>[4x]MAKKTSSKGKLPPGPTPLPFIGNYLQLNTEQMYNSLMKISERYGPVFTIHLGPRRVVVLCGHDAVREALVDQAEEFSGRGEQATFDWVFKGYGVVFSNGERAKQLRRFSIATLRDFGVGKRGIEERIQEEAGFLIDALRGTGGANIDPTFFLSRTVSNVISSIVFGDRFDYKDKEFLSLLRMMLGIFQFTSTSTGQLYEMFSSVM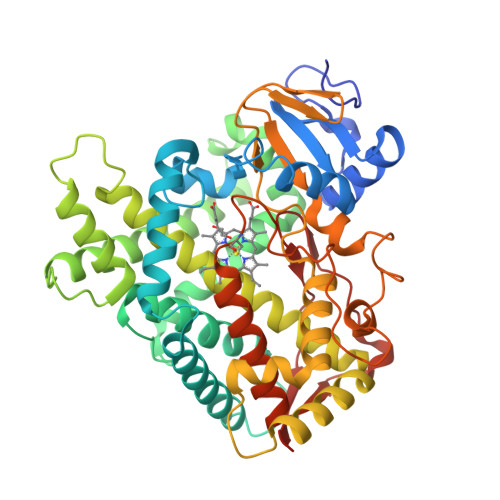KHLPGPQQQAFQLLQGLEDFIAKKVEHNQRTLDPNSPRDFIDSFLIRMQEEEKNPNTEFYLKNLVMTTLQLFIGGTETVSTTLRYGFLLLMKHPEVEAKVHEEIDRVIGKNRQPKFEDRAKMPYMEAVIHEIQRFGDVIPMSLARRVKKDTKFRDFFLPKGTEVYPMLGSVLRDPSFFSNPQDFNPQHFLNEKGQFKKSDAFVPFSIGKRNCFGEGLARMELFLFFTTVMQNFRLKSSQSPKDIDVSPKHVGFATIPRNYTMSFLPRHHHH2-deoxy-2-fluoro-alpha-D-mannopyranose | C6 H11 F O5 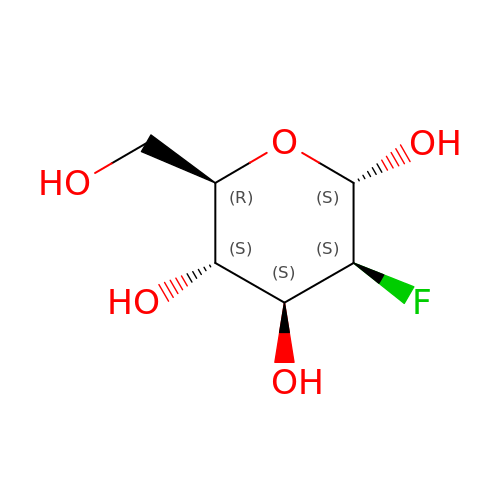| ZCXUVYAZINUVJD-AIECOIEWSA-N The Polo-like kinases (PLKs 1-5) are a family of serine/threonine protein kinases essential for cell cycle regulation and cell proliferation. In humans, PLK1 regulates key processes during cell division, including mitotic entry, spindle formation, chromosome segregation, and cytokinesis. PLK1 inhibitors target either the N-terminal catalytic kinase domain (KD) with ATP-binding sites or the C-terminal polo-box domain (PBD), which mediates interactions with phosphorylated substrates. Among them, PLK1 is an attractive anticancer drug target owing to its overexpression in various human cancers.

We designed and developed NC1, a PROTAC combining PLK1-targeting inhibitor 4j and UBR-box-targeting ligand Arg12, acting as an N-end rule pathway or N-degron inhibitor. Among the PLHSpT derivatives, PLH(n-octylphenyl)SpT (4j) is the most potent PLK1 PBD inhibitor. To further confirm PLK1 degradation resulted from selective binding of PLK1 PBD and UBR ligands in NC1 via ternary complex formation, the crystal PROTAC structure complexed with PLK1 PBD was investigated. The PLK1 PBD ligand in the PROTAC interacted similar to the potent pentapeptide, PLH(n-octylphenyl)SpT (4j) within the PBD crystal lattice. For example, the pyrrolidine in the PLK1 warhead of the PROTAC interacted with Phe535, Trp414, and Arg518 within the pyrrolidine binding pocket. Additionally, the long alkylphenyl chain at the histidine residue penetrated via a deep, conserved hydrophobic channel formed by tyrosine residues. The phosphate group of pT engaged in polar interactions with His538 and Lys540 within the phosphate binding pocket. Furthermore, an overlay view of the newly synthesized NC1 with PLH(n-octylphenyl)SpT (4j) confirmed that the ligands project toward the binding pockets and interact with residues in a similar pattern. This finding showed that the PLK1 ligand in the PROTAC is capable of reaching its target and maintaining activity, even when integrated with a linker and an E3 ligase ligand. The crystal structure of the PBD-NC1 complex identified key PLK1 PBD binding interactions and isothermal titration calorimetry (ITC) confirmed a binding affinity of 6.06 µM between NC1 and PLK1 PBD.

> CHLSDLLQQLTSVNASKPSERGLVRQEEAEDPACIPIFWVSKWVDYSDKYGLGYQLCDNSVGVLFNDSTRLILYNDGDSLQYIERDGTESYLTVSSHPNSLMKKITLLNYFRNYMSEHLLKAGANITPREGDELARLPYLRTWFRTRSAIILHLSNGTVQINFFQDHTKLILCPLMAAVTYINEKRDFQTYRLSLLEEYGCCKELASRLRYARTMVDKLLSSRS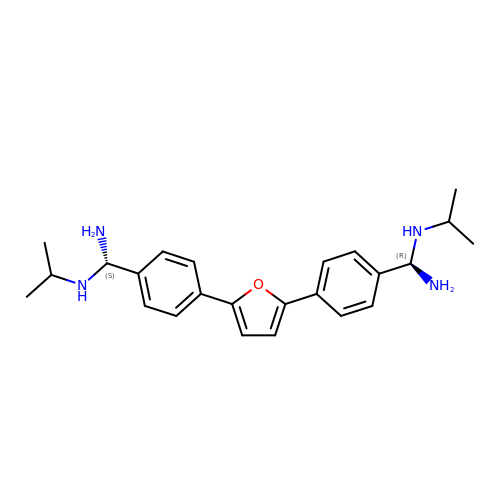2,5-BIS{[4-(N-ISOPROPYL)DIAMINOMETHYL]PHENYL}FURAN | C24 H32 N4 O | MLUJKSDBDBJFEG-PSWAGMNNSA-N> SNADSLPERIDLFVSLFDYNSATTSYDIRSIQTDFPTRLLTPDSMLPQTSEYPLKDIQLLYKLAQSCTGKLPLSPLITEPLVFTRSLCKGSSLSPRWFARSG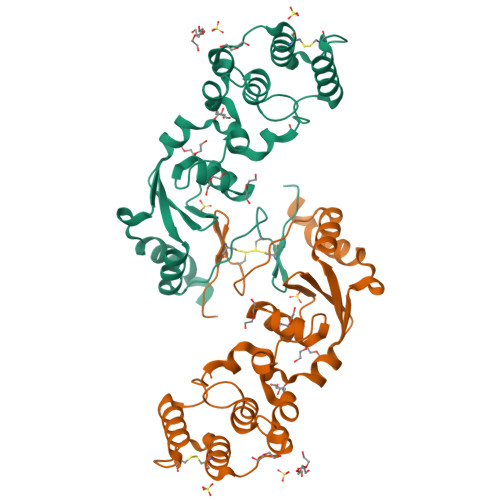LIHPGGGTYAFRYAEKYPAQFANLLPYMHIQERPNAAEGTLLYHLQNMGEDAINALVSGASMFGSGSDLWLRKGDIYYLFNEETWLTNANKAGLSYSLLSADTCFIQRGNICWDVEDHS>[9x]MEFTVSTTEDLQRYRTECVSSLNIPADYVEKFKKWEFPEDDTTMCYIKCVFNKMQLFDDTEGPLVDNLVHQLAHGRDAEEVRTEVLKCVDKNTDNNACHWAFRGFKCFQKNNLSLIKASIKKD

Ae. aegypti OBP22 (AeOBP22) is a member of the OBP family of proteins that has been directly implicated in regulating these feeding behaviors. AeOBP22 is unusual in that it is expressed in multiple chemosensory tissues, including in the antenna, the proboscis of the females, the thoracic spiracles, in the male reproductive glands where it is transferred to the females during mating, and in the salivary glands. The monomeric forms of AeOBP22 are similar to other classical OBPs which consist of six α-helices stabilized by three disulfide bridges surrounding a hydrophobic pocket. Our results provide evidence that fatty acids are likely natural ligands for AeOBP22 and that the binding of long-chain fatty acids (C15-C20) is enhanced by a conformational change in the C-terminal tail that is critical to generate a high affinity binding site.

The second crystal form was solved in the P31 space group and contains nine molecules in the asymmetric unit arranged in a pseudo three-fold arrangement of “trimers” consisting of domain swapped dimer and a separately packed monomer. The dimers are identical to those observed in crystal form 1 and superimpose with an average pairwise RMSD of 0.47 Å. The individual monomers superimpose to each other with an average pairwise RMSD of ~0.2 Å. Ligands are observed bound at the center of each monomer with residues 112–121 forming an α-helix that forms one edge of the ligand-binding pocket. No ligand is observed in the dimeric components. In this form we solved the structures with palmitic acid (C16:0), palmitoleic acid (C16:1), and eicosanoic acid (C20) complexes. Saturated C16 binds weakly with KD ~690 nM, however, introduction of a single degree of unsaturation at the Δ9 position (C16:1) leads to an approximate four-fold increase in the binding affinity (KD = 175 ± 41 nM). Dodecanoic acid and palmitoleic acid are strong oviposition attractants in Ae. aegypti, whilst the saturated C14–C16 and C18 acids are attractants at low concentrations but repellents at high concentrations. Therefore, we conclude that the domain swapped dimers are an artifact of the crystallization process, and further discussions below are confined to the structures of the monomeric forms.SHMTs are α-class pyridoxal 5′-phosphate (PLP)-dependent enzymes which transfer hydroxymethyl of Ser to – typically polyglutamylated (polyGlu) – tetrahydrofolate (H4PteGlun), producing Gly and 5,10-CH2-H4PteGlun. Here we report crystal structures of a chloroplastic SHMT enzyme from the model legume plant, Medicago truncatula (Mt), which similarly to At has seven SHMT isoforms. MtSHMT3 is a member of the α-class of PLP enzymes, and its overall fold is typical for this family. A subunit of MtSHMT3 can be subdivided into three regions: N-terminal arm, large domain, and small domain, consistently with other SHMTs.

The holo/apo structure of MtSHMT3, with one tetramer in the crystallographic asymmetric unit, shows two states, with and without the PLP prosthetic group. More precisely, two protein chains (A and B) contain the PLP bound as a Schiff base internal aldimine to K318 (holo-state) with full occupancy. In one chain there is no cofactor bound (chain C, apo-state), whereas in the chain D, PLP is present at a partial occupancy. Notably, no additional PLP was added during the protein expression or purification, thus the prosthetic group originates solely from the culture. Comparison of MtSHMT3 subunits in apo- and holo-states revealed that a fragment of the protein undergoes significant rearrangements upon PLP binding. Binding of PLP in one MtSHMT3 subunit is accompanied by conformational changes within residues 133–151 of the other subunit of the tight dimer. With PLP bound in subunit A, the peptide bond L138-P139 in subunit B is in trans-conformation, and the helix α5 gains an additional twist to start from E148 – leaving only residues 133–147 in the loop region (orange). Two of the loop residues, Y134∗ and E136∗ (an asterisk indicates a residue from the other subunit of the tight, obligate dimer) hydrogen-bond PLP in the dimer mate (see below), which is likely the reason that drives such disorder-to-order transition. An extensive network of non-covalent interactions secures PLP internal aldimine in the large domain of MtSHMT3. Overall, the environment of R454 guanidinium group is a good placeholder for a carboxylic group, as it binds an acetate anion in the holo-MtSHMT3 structure. Binding of PLP is accompanied by a local disorder-to-order transition but does not involve large rearrangements, such as those observed in hmSMHT2.

>[4x]SNAFLDYGLSEADPDVHAIINKEKDRQFRSLELIASENFTSKAVMEAVGSCLTNKYSEGLPGKRYYGGNEHIDELEILCQQRALAAFHLDGDKWGVNVQPLSGSPANFAVYTAILKPHDRIMGLDLPHGGHLSHGFMTAKRRVSGTSIYFESMPYRLDESTGVIDYDMLEKTAALFRPKLIIAGASAYPRDIDYARFRKIADSVGAFLMMDMAHVSGLIAASVLADPFEFVDIVTTTTHKSLRGPRGGMIFFKKDAVHGVDLESAINNAVFPGLQGGPHNHTIGGLAVCLKYAQSPDFKNYQNQVVANCRALANRLVEHEYKLVSGGSDNHLVLVDLRPSGIDGARVEKILDMASITLNKNSVPGDKSALVPGGIRIGSPAMTTRGLGEKEFELIADLIHEGVRISLEAKSLVSGTKVQDFLNFVLAPEFPLGDKVSNLRRKVEALATQYPIPGV> MAMLPPPGPQSFVHFTKQSLALIEQRIAERKSKEPKEEKKDDDEEAPKPSSDLEAGKQLPFIYGDIPPGMVSEPLEDLDPYYADKKTFIVLNKGKTIFRFNATPALYMLSPFSPLRRISIKILVHSLFSMLIMCTILTNCIFMTMNNPPDWTKNVEYTFTGIYTFESLVKILARGFCVGEFTFLRDPWNWLDFVVIVFAYLTEFVNLGNVSALRTFRVLRALKTISVIPGLKTIVGALIQSVKKLSDVMILTVFCLSVFALIGLQLFMGNLKHKCFRNSLENNETLESIMNTLESEEDFRKYFYYLEGSKDALLCGFSTDSGQCPEGYTCVKIGRNPDYGYTSFDTFSWAFLALFRLMTQDYWENLYQQTLRAAGKTYMIFFVVVIFLGSFYLINLILAVVAMAYEEQNQANIEEAKQKELEFQQMLDRLKKEQEEAEAIAAAAAEYTSIRRSRIMGLSESSSETSKLSSKSAKERRNRRKKKNQKKLSSGEEKGDAEKLSKSESEDSIRRKSFHLGVEGHRRAHEKRLSTPNQSPLSIRGSLFSARRSSRTSLFSFKGRGRDIGSETEFADDEHSIFGDNESRRGSLFVPHRPQERRSSNISQASRSPPMLPVNGKMHSAVDCNGVVSLVDGRSALMLPNGQLLPEVIIDKATSDDSGTTNQIHKKRRCSSYLLSEDMLNDPNLRQRAMSRASILTNTVEELEESRQKCPPWWYRFAHKFLIWNCSPYWIKFKKCIYFIVMDPFVDLAITICIVLNTLFMAMEHHPMTEEFKNVLAIGNLVFTGIFAAEMVLKLIAMDPYEYFQVGWNIFDSLIVTLSLVELFLADVEGLSVLRSFRLLRVFKLAKSWPTLNMLIKIIGNSVGALGNLTLVLAIIVFIFAVVGMQLFGKSYKECVCKINDDCTLPRWHMNDFFHSFLIVFRVLCGEWIETMWDCMEVAGQAMCLIVYMMVMVIGNLVVLNLFLALLLSSFSSDNLTAIEEDPDANNLQIAVTRIKKGINYVKQTLREFILKAFSKKPKISREIRQAEDLNTKKENYISNHTLAEMSKGHNFLKEKDKISGFGSSVDKHLMEDSDGQSFIHNPSLTVTVPIAPGESDLENMNAEELSSDSDSEYSKVRLNRSSSSECSTVDNPLPGEGEEAEAEPMNSDEPEACFTDGCVWRFSCCQVNIESGKGKIWWNIRKTCYKIVEHSWFESFIVLMILLSSGALAFEDIYIERKKTIKIILEYADKIFTYIFILEMLLKWIAYGYKTYFTNAWCWLDFLIVDVSLVTLVANTLGYSDLGPIKSLRTLRALRPLRALSRFEGMRVVVNALIGAIPSIMNVLLVCLIFWLIFSIMGVNLFAGKFYECINTTDGSRFPASQVPNRSECFALMNVSQNVRWKNLKVNFDNVGLGYLSLLQVATFKGWTIIMYAAVDSVNVDKQPKYEYSLYMYIYFVVFIIFGSFFTLNLFIGVIIDNFNQQKKKLGGQDIFMTEEQKKYYNAMKKLGSKKPQKPIPRPGNKIQGCIFDLVTNQAFDISIMVLICLNMVTMMVEKEGQSQHMTEVLYWINVVFIILFTGECVLKLISLRHYYFTVGWNIFDFVVVIISIVGMFLADLIETYFVSPTLFRVIRLARIGRILRLVKGAKGIRTLLFALMMSLPALFNIGLLLFLVMFIYAIFGMSNFAYVKKEDGINDMFNFETFGNSMICLFQITTSAGWDGLLAPILNSKPPDCDPKKVHPGSSVEGDCGNPSVGIFYFVSYIIISFLVVVNMYIAVILENFSVATEESTEPLSEDDFEMFYEVWEKFDPDATQFIEFSKLSDFAAALDPPLLIAKPNKVQLIAMDLPMVSGDRIHCLDILFAFTKRVLGESGEMDSLRSQMEERFMSANPSKVSYEPITTTLKRKQEDVSATVIQRAYRRYRLRQNVKNISSIYIKDGDRDDDLLNKKDMAFDNVNENSSPEKTDATSSTTSPPSYDSVTKPDKEKYEQDRTEKEDKGKDSKESKK;> MGRLLALVVGAALVSSACGGCVEVDSETEAVYGMTFKILCISCKRRSETNAETFTEWTFRQKGTEEFVKILRYENEVLQLEEDERFEGRVVWNGSRGTKDLQDLSIFITNVTYNHSGDYECHVYRLLFFENYEHNTSVVKKIHIEVVDKANRDMASIVSEIMMYVLIVVLTIWLVAEMIYCYKKIAAATETAAQENASEYLAITSESKENCTGVQVAE;> MHRDAWLPRPAFSLTGLSLFFSLVPPGRSMEVTVPATLNVLNGSDARLPCTFNSCYTVNHKQFSLNWTYQECNNCSEEMFLQFRMKIINLKLERFQDRVEFSGNPSKYDVSVMLRNVQPEDEGIYNCYIMNPPDRHRGHGKIHLQVLMEEPPERDSTVAVIVGASVGGFLAVVILVLMVVKCVRRKKEQKLSTDDLKTEEEGKTDGEGNPDDGAK

Voltage-gated sodium (Nav) channels govern membrane excitability in neurons and muscles. Nav1.7, encoded by SCN9A and primarily localized to the dorsal root ganglion neurons, has been explored as a prominent target for pain management. The S1-S4 segments in each repeat constitute the flanking voltage-sensing domain (VSD), and the S5-S6 segments enclose the PD that is responsible for selective and gated ion permeation. Here we report high-resolution cryo-EM structures of human Nav1.7 treated with drugs and lead compounds with representative chemical backbones at resolutions of 2.6-3.2 Å.

Unexpectedly, LCM has a second binding pose that directly plugs into the selectivity filter from the central cavity. We will discuss the second site in a later session. For illustration simplicity, we will name LCM as LCM-1 and LCM-2 in site BIG and the central cavity, respectively. The amide nitrogen from the central amide group of LCM-1 is H-bonded with the carboxyl group of Glu406 on S6I, and the carbonyl oxygen of CBZ receives an H-bond from Asn1461 on S6III. Beneath the ceiling of the central cavity, the Y-shaped LCM-2 is positioned off the central axis, closer to repeats I and IV. The benzyl ring is embedded in a pocket enclosed by residues Ser1697, Ile1744, Phe1748, Val1751, and Val1752. The two amides are H-bonded to the backbone carbonyl group of Thr1696 on the P1 loop of repeat IV, forming a stable anchor for LCM-2. The carbonyl oxygen from the acetylamino moiety interacts with Lys1406, which is one constituent of the DEKA motif on repeat III, and the amide nitrogen engages in an H-bond with Gln360, which is stabilized by the side chain hydroxyl group of Ser390. The extensive H-bond network may account for the stronger density of LCM-2 than that of LCM-1. Based on this classification, LCM-2 binds to site UC.>[3x]GHSMHHHHHHLGNKLSISDLKDIKNKKVLVRVDFNVPIENGIIKDTNRITATLPTINHLKKEGASKIILISHCGRPDGLRNEKYTLKPVAETLKGLLGEEVLF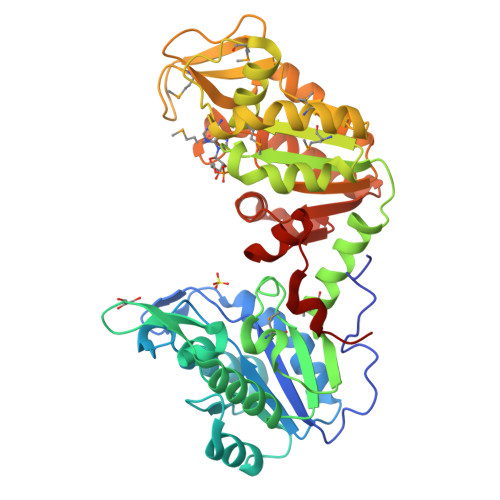LNDCVGKEVEDKINAAKENSVILLENLRFHIEEEGKGVDANGNKVKANKEDVEKFQNDLTKLADVFINDAFGTAHRAHSSMVGVKLNVKASGFLMKKELEYFSKALENPQRPLLAILGGAKVSDKIQLIKNLLDKVDRMIIGGGMAYTFKKVLNNMKIGTSLFDEAGSKIVGEIMEKAKAKNVQIFLPVDFKIADNFDNNANTKFVTDEEGIPDNWMGLDAGPKSIENYKDVILTSKTVIWNGPQGVFEMPNFAKGSIECLNLVVEVTKKGAITIVGGGDTASLVEQQNKKNEISHVSTGGGASLELLEGKELPGVLALSNK> KETAAAKFERQHMDSSTS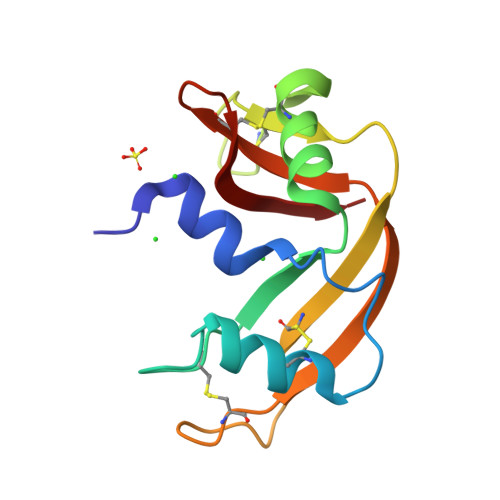AASSSNYCNQMMKSRNLTKDRCKPVNTFVHESLADAQAVCSQKNVACKNGQTNCYQSYSTMSITDCRETGSSKYPNCAYKTTQANKHIIVACEGNPYVPVHFDASV>MIKKCLFPAAGYGTRFLPITKTIPKEMLPIVDKPLIQYAVEEAMEAGCEVMAIVTGRNKRSLEDYFDTSYEIEHQIQGTNKENALKSIRNIIEKCCFSYVRQKQMKGLGHAILTGEALIGNEPFAVILADDLCISHDHPSVLKQMTSLYQKYQCSIVAIEEVALEEVSKYGVIRGEWLEEGVYEIKDMVEKPNQEDAPSNLAVIGRYILTPDIFEILSETKPGKNNEIQITDALRTQAKRKRIIAYQFKGKRYDCGSVEGYIEASNAYY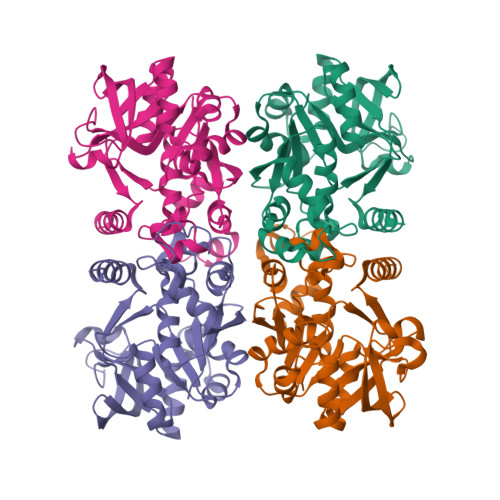KKRLLEHHHHHH[4x]>MCGNNMSTPLPAIVPAARKATAAVIFLHGLGDTGHGWAEAFAGIRSSHIKYICPHAPVRPVTLNMNVAMPSWFDIIGLSPDSQEDESGIKQAAENIKALIDQEVKNGIPSNRIILGGFSQGGALSLYTALTTQQKLAGVTALSCWLPLRASFPQGPIGGANRDISILQCHGDCDPLVPLMFGSLTVEKLKTLVNPANV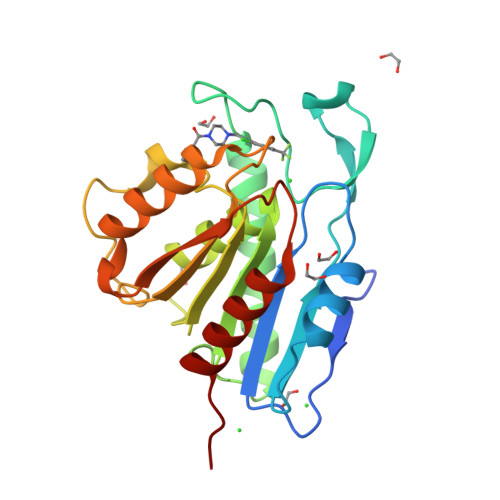TFKTYEGMMHSSCQQEMMDVKQFIDKLLPPID[2x]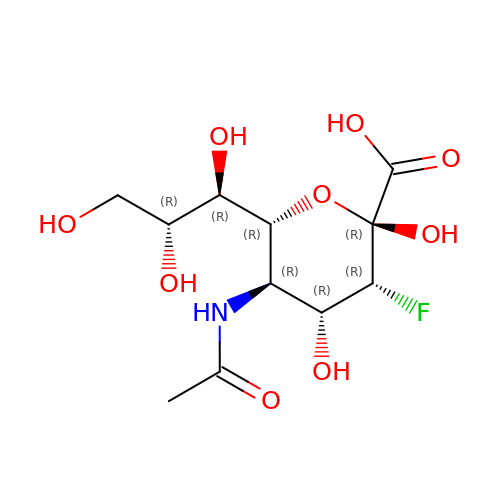5-acetamido-3,5-dideoxy-3-fluoro-D-erythro-alpha-L-manno-non-2-ulopyranosonic acid | C11 H18 F N O9 | ALJLGESFXXDPKH-RISWTRDCSA-N> GADRTLRRMRKVVNIINAMEPEMEKLSDEELKGKTAEFRARLAAGAVLENLIPEAFAVVREASKRVFGMRHFDVQLLGGMVLNERCIAEMRTGEGKTLTATLPAYLNALTGKGVHVVTVNDYLAQRDAENNRPLFEFLGLTVGINLPGMPAPAKREAYAADITYGTNNEYGFDYLRDNMAFSPAARVQRKLHYALVDEVDSILIDEARTPLIISGPAEDSSEMYKRVNKIIPHLIRQEKEDSETFQGEGHFSVDEKSRQVNLTERGLVLIEELLVKEGIMDEGESLYSPANIMLMHHVTAALRAHALFTRDVDYIVKDGEVIIVDEHTGRTMQGRRWSDGLHQAVEAKEGVQIQNENQTLASITFQNYFRLYEKLAGMTGTADTEAFEFSSIYKLDTVVVPTNRPMIRKDLPDLVYMTEAEKIQAIIEDIKERTAKGQPVLVGTISIEKSELVSNELTKAGIKHNVLNAKFHANEAAIVAQAGYPAAVTIATNMAG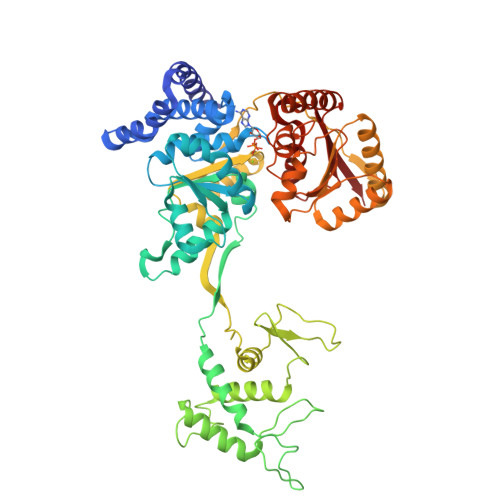RGTDIVLGGSWQAEVAALENPTAEQIEKIKADWQVRHDAVLEAGGLHIIGTERHESRRIDNQLRGRSGRQGDAGSSRFYLSM6-methyl-~{N}-(4-methylsulfonylphenyl)thieno[2,3-d]pyrimidin-4-amine | C14 H13 N3 O2 S2 | 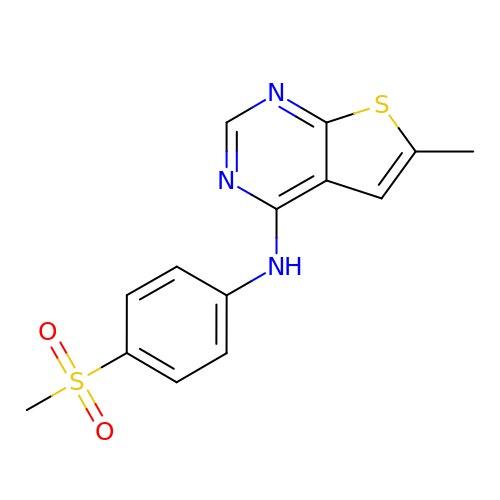QVQHWPLHUNEREE-UHFFFAOYSA-N>[2x]MKEITLTIDGKVCKGVQGDTILDVANKNDVYIPTLCYQKGLTPIGACRMCVVQLEGNPKMLPSCTTPAQDGMVVVTKNEKLKDYRRQILELLFAGRNHFCMYCSQSGDCELQRLAIEHEMDSVRFPYLYEDFEVDATDPNLMMDHNRCVLCQRCIRTCSEIVGAHTLDLERRGWQAKVIADLGKRLRESDTCVNCGACAQSCPTGTITIREFAYRGRRSECDAVVESVCPLCAVGCKIKTYVRTGSIVRVEGTGVEEPDGGQLCHMGRWWLPESTERERVTVPLIREGASYREATWEEALALASAEFKKAYDQEKAGAILSSLCTDEELTLFSALFRNALKMKHIDTFDGDIIRGFFKGFMPFREQGVRPFTAAHHILDSDLIITMFADPQKEAPVVASYIRVACLHRNAKLMNLSYGPSPFPGLVDLDIRLPEGQAVPKALSNLAEIIGKISLGPSDMASFGEFEAGAGKALSSYRESIEESARAMGLDPKIAEEVALMLISARRPIFIIGGRATKSHELVTAACNLAVASKAFFEDGLGVVPLLVSANSLGARNTVVSENPWLGRERRDFLYVFSTAMVPEEEEILAAISATRFVVVQTPFKVRPLVNLADILLPAPAWYERSGHFCTIEGERRKLNTIVPPKGEIKSLHYVMDEFAKKLGVKLERPEVSPCEEIFKSQLRASEARIVTL;>[2x]MAIYRAHVLVCRGTGCTASGAPGVMKAFKEELAKKGLDREVMLVETGCHGMCEMGPVVVVYPEGAFYCRVTPEDVPEIVEEHLYKGRIVQRLLYTVPEDMEKVPYYKDIPFYSKQHRIVLSNCGYIDPEKIEEYIARDGYMALGKALLEMTPEEVLEEVKKSGLRGRGGAGFPTGLKWEFAKKASGDKKYVICNADEGDPGAFMDRSTLEGDPHSVIEGMTIGAYVIGADEGYIYCRAEYPLAIKRLKIAIAQAEEMGLLGDHIMGTNFSFHLHLKEGAGAFVCGEETALMASIEGRRGMPRPRPPFPAQHGLWGKPTNINNVETWANVPRIILNGADWFASMGTEKSKGTKIFALTGKITNTGLIEVPMGITIREIIYELGGGILNGKEFKAVQIGGPSGGCLTKEHLDLPIDYESLTAAGAIMGSGGLVVMDEDTCMVDVAKFFLEFTQRESCGKCVPCREGTKQMLLMLQKICNGEGTMDDLSKLEELAHMVKETSLCGLGQTAPNPVITTIRYFRDEYVAHIKDKRCPAKICPALIKYVVDPEKCRKCGLCARNCPVKCISGDRQTPYLINQEKCIKCGTCMQVCPFGAIGKV;>MALSTVDVVEKVKEIVAPWKGKQGGLIPILQEVQRELGYLPEEALLTISRELKMPKAEVYGVATFYAQFHLKPRGRHVIRVCRGTACHVRGSLQILEKVKQMLGIEENETTDDLRFTLEPVACLGACGLAPVMMVDEDTHGRMTPDKIQAILDKYQ[2x];>MTEVFKLEINPVTRIEGHGKITVMLDESGHVRETRFHVTQYRGFEVFTHGRDFREMPVITPRICGICPVSHHLASAKACDEILGVTITPAAHKLRELMHMGQIVQSHALSFFHLSSPDILWGFDAPVKIRNVAGLVDRYPELAKKGIMLRKFGQEIIKTLGGKKIHPWHSIPGGVNRSLTPQERDAIAAQLPEMKSIAMEAIKLIKDYLQEGGEELKEFATLDTAYMGLVRDGYLELYDGEVRIKAPRGRILDQFDPKDYLDHIGEHVEPWSYLKFPFYKALGFPHGSYRVGPLARLNAADAVSTPEASKEFALYKEMGEDGIVPYTLYYHYARLIEALYGLERIEQLLADPDITSSDLRVTSKEINPEGIGVIEAPRGTLIHHYQVNESGVITKVNLIVATGHNNFAMNKGVEMVAKKYITGTNVPEGVFNRLEHVIRAYDPCLSCSTHAVGKMPLKLELVGPTGEILKEVTRD[2x];>MAKAKVATFWLEACAGCHMSFLDLDERLIDLFQNVEILFSPIVDAKDIPNIDVGVLSGGLGNVEEVELAKKMRERCKYLVAWGDCAVFGGINCMRNFIPKDVVLREGYIETASTVNPQGIVPSEDIPELLPRALPIDYEVKVDVYVPGCPPDADTIYYVFKELLAGRVPKVPSEMMRYD[2x]

In summary, we have described the cryo-EM structure of NiFe-HydABCSL, an electron-bifurcating hydrogenase consisting of a conventional NiFe-hydrogenase module (SL subunits) and of a bifurcating module (ABC subunits) that is highly similar to a previously characterized bifurcating heterotrimeric FeFe-hydrogenase. We report cryo-EM structures of the related NiFe-HydABCSL hydrogenase that reversibly oxidizes H2 and couples endergonic reduction of ferredoxin with exergonic reduction of NAD. Here, we report cryo–electron microscopy (cryo-EM) structures of NiFe-HydABCSL determined in a flavin-free apo state, in an “electron bifurcation-ready” (BR) state, and in a “post-electron bifurcation” (PB) state. The structures of the NiFe-enzyme show that none of the previous proposals for the site of bifurcation in [FeFe]-HydABC hydrogenases are likely to be correct and that instead electron bifurcation occurs at a single NAD(H)-binding flavin in combination with a unique arrangement of three iron-sulfur clusters.

To understand the electron transfer pathways in the NiFe-enzyme, we prepared cryo-EM grids in the presence of purified A. mobile Fd, FMN, and NADH. Fd was not resolved in the 3D map, perhaps because Fd binds only transiently. The structure is similar to that of the apo state, but the HydC Fd-like CTD and the HydB NTD, which were well resolved in the flavin-free apo state, became invisible in the high-resolution EM map. It is likely that the FMN and NADH binding caused a series of structural changes leading to the release of HydB NTD and HydC CTD from the main body of the structure and becoming flexible. FMN and NADH had well-defined densities in HydB and are stacked in parallel to each other in a configuration that resembles those in Nqo1 of complex I. Compared to the apo state, all the FMN/NAD-coordinating loops underwent substantial conformational changes to accommodate the two cofactors. The distance between the NAD nicotinamide C4 atom and the ionizable N5 atom in the FMN isoalloxazine ring is only 4.2 Å, well within the hydride transfer range. The FMN isoalloxazine ring is 6.0 Å from the B1 [4Fe-4S] cluster, providing an electron transfer path from FMN and the NiFe site via the chain of five clusters B1-A1-A2-A3-S1. Because it sits at the meeting point of the NiFe-S1-A3-A2-A1-B1 and B5-B4-B3-B2-C1 pathways, the single-flavin FMN must play, at least in part, the role of electron bifurcation. In the active state when both NAD and FMN are bound, we found that HydC CTD becomes mobile and interconverts between a bifurcation-ready BR state where electron transfer from FMN to the C1 [2Fe-2S] is permitted and a post-bifurcation PB state where electron transfer from C1 to B2 [2Fe-2S] is permitted.>MTDLKASSLRALKLMDLSTLNGDYTDEKVIALCHQAKTPVGNTAAISIYPRSIPIARKTLKEQGTPEIRIATVTNFPHGNDDIEIALAETRAAIAYGADEVDVVFPYRALMAGNEQVGFDLVKACKEACAAANVLLKVIIESGELKDEALIRKASEISIKAGADFIKTSTGLVAVNATPESARIMMEVIRDMGVEKSVGFKVTGGARTAEDAQKYLAIADELFGA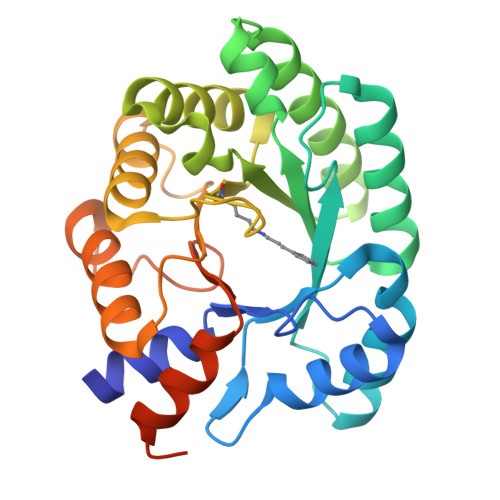DWADARHYRFGASGLLASLLKALGHGDGKSASSYLEHHHHHH[12x]> APNLAGAVEFNDVKTLLREWITTISDPMEEDILQVVKYCTDLIEEKDLEKLDLVIKYMKRLMQQSVESVWNMAFDFILDNVQ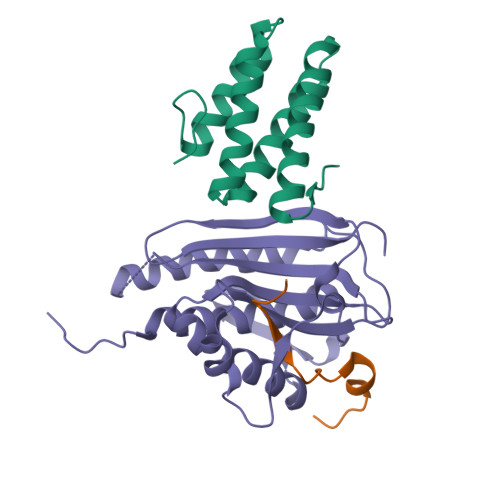VVLQQTYGSTLKVT;> RTANILKPLMSPPSREEIMATLL;> TQDLNFGQVVADVLCEFLEVAVHLILYVREVYPVGIFQKRKKYNVPVQMSCHPELNQYIQDTLHCVKPLLEKNDVEKVVVVILDKEHRPVEKFVFEITQPPLLSISSDSLLSHVEQLLRAFILKISVCDAVLDHNPPGCTFTVLVHTREAATRNMEKIQVIKDFPWILADEQDVHMHDPRLIPLKTMTSDILKMQLYVEERAHK Here, we report the composition, structure and function of the type I-G Cascade CRISPR effector from Thioalkalivibrio sulfidiphilus, revealing key new molecular details. The unique Csb2 subunit processes pre-crRNA, remaining bound to the 3′ end of the mature crRNA, and seven Cas7 subunits form the backbone of the effector. Cas3 associates stably with the effector complex via the Cas8g subunit and is important for target DNA recognition. Structural analysis by cryo-Electron Microscopy reveals a strikingly curved backbone conformation with Cas8g spanning the belly of the structure.

The large subunit of type I-G systems has no detectable sequence identity to any other Cas8 protein. We predicted the structure using AF2, which gave strong support for an extended structure with a mixed (α + β) N-terminal domain and a helical C-terminal domain. Thus, structure predictions suggest that Cas8g is a highly divergent member of the Cas8 family with a C-terminal Cas11-like domain. A poorly defined elongated density that runs across the belly of the Cas7-crRNA crescent complex structure was observed in our CryoEM reconstruction. The density resembled a bi-lobed structure with a larger head closer to the 5′ crRNA end and with predominant interactions with the first two Cas7 proteins. Using multibody reconstruction in RELION 4 incorporating intrinsic motion we were able to improve the overall quality of the density to ∼8 Å resolution. The enhanced map enabled us to model the Cas8g subunit using the AF2 predicted structure as starting model. We separated the N- and C-terminal into separate rigid bodies and using DockEM we modelled the overall structure of the bound Cas8g protein. The Cas8g subunit is clearly flexible and consequently is observed at only low resolution. The N-terminal domain of Cas8g sits a considerable distance from the 5′ end of the crRNA, and this together with the lack of a Cas5 subunit represents a significant point of divergence from the other structures.

> MDKDMHINEIVLRGCAPTPLAAYLKALGVLRLVCEQVDATAKGWWQDECFMLRTRLDDNDLRRFFIEDYRPTPMLSPWNGGSGFYRKGNETAWSTLEKIITTQAERWRPFRDTAEVMADALEHLKLTEKPAELDKRALLARLRATLDDEFLPWLDAAVLLTDDKPDYPPLLGTGGNDGRLDFTSNYMQRLLEMFDPVTGKAQGDVGNKLESALFARPVPGMTALAIGQFSPGAAGGPNSSTGFDSGAQVNIWDYVLMLEGALLFAATATRRLESADPSALSYPFTVRPSGGGSGAVALGDERPARAEIWMPLWERPASLPELRVLLGEGRVTLNGRLPRDGLDFARAVAKLGTDRGVRAFQRYAFMMRSGKAYLATPLNRFHVHRNPKADLIDQLERGDWLRRFRRAARSTHAPARLQGLAHRLDDALFDLVRVADPRRVQEVLKVLGEVQFYLALSPSLREQVRPVPRLDAHWVEAARDDSHEFRVAAALAGLDDGLPMGVHLAPIDPVKRNVWAPESRLAVWGQGNLSDNLAQVLQRRLLTASRTDLNDKPLSGRCPADEGAVAAFLAGDADERRIAELMAGLACARLPARLPLRQRGASEASSLPMIYALLKPLFVPDAQLREAAVLTPDGCLPLPPALPRLLRAGPAGVGRAVDLARRRRRASGLADAGWRLTPPYPDGGRLLAALMIPVEIRVIKGFIKRLADHKSDEPATQDAS>SNAMRETVEIMRYPVTLTPAPEGGYMV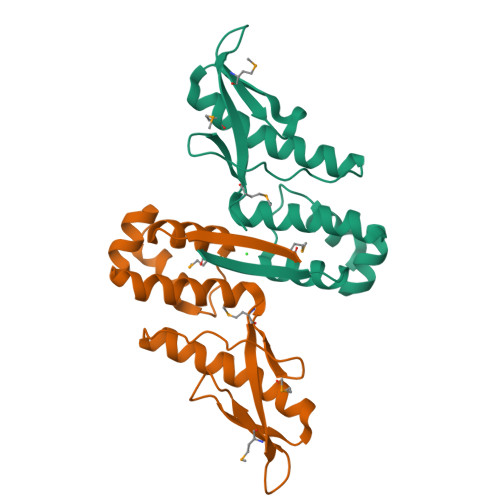SFVDIPEALTQGETVAEAMEAAKDALLTAFDFYFEDNELIPLPSPLNSHDHFIEVPLSVASKVLLLNAFLQSEITQQELARRIGKPKQEITRLFNLHHATKIDAVQLAAKALGKELSLVMV[4x]> MG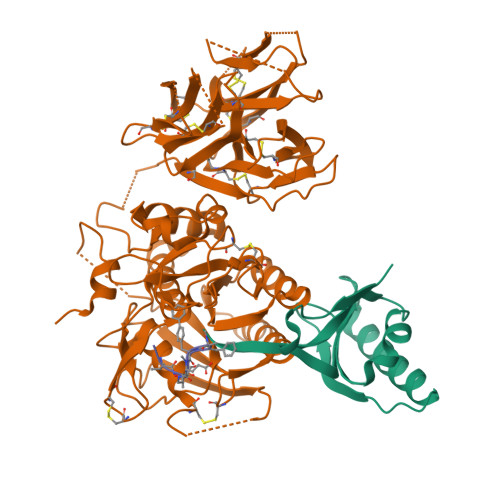TVSSRRSWWPLPLLLLLLLLLGPAGARAQEDEDGDYEELVLALRSEEDGLAEAPEHGTTATFHRCAKDPWRLPGTYVVVLKEETHLSQSERTARRLQAQAARRGYLTKILHVFHGLLPGFLVKMSGDLLELALKLPHVDYIEEDSSVFAQ;> SIPWNLERITPPRYRADEYQPPDGGSLVEVYLLDTSIQSDHREIEGRVMVTDFENVPEEDGTRFHRQASKCDSHGTHLAGVVSGRDAGVAKGASMRSLRVLNCQGKGTVSGTLIGLEFIRKSQLVQPVGPLVVLLPLAGGYSRVLNAACQRLARAGVVLVTAAGNFRDDACLYSPASAPEVITVGATNAQDQPVTLGTLGTNFGRCVDLFAPGEDIIGASSDCSTCFVSQSGTSQAAAHVAGIAAMMLSAEPELTLAELRQRLIHFSAKDVINEAWFPEDQRVLTPNLVAALPPSTHGAGWQLFCRTVWSAHSGPTRMATAIARCAPDEELLSCSSFSRSGKRRGERMEAQGGKLVCRAHNAFGGEGVYAIARCCLLPQANCSVHTAPPAEASMGTRVHCHQQGHVLTGCSSHWEVEDLGTHKPPVLRPRGQPNQCVGHREASIHASCCHAPGLECKVKEHGIPAPQEQVTVACEEGWTLTGCSALPGTSHVLGAYAVDNTCVVRSRDVSTTGSTSEEAVTAVAICCRSRHLAQASQELQ;> XFVATTFAFX>TGRPEWIWLALGTALMGLGTLYFLVKGMGVSDPDAKKFYAISTLVPAIAFTMYLSMLLGYGLTMVPFGGEQNPIYWARYADWLFTTPLLLLDLALLVDADQGTILALVGADGIMIGTGLVGALTKVYSYRFVWWAISTAAMLYILYVLFFGFTSKAESMRPEVASTFKVLRNVTVVLWSAYPVVW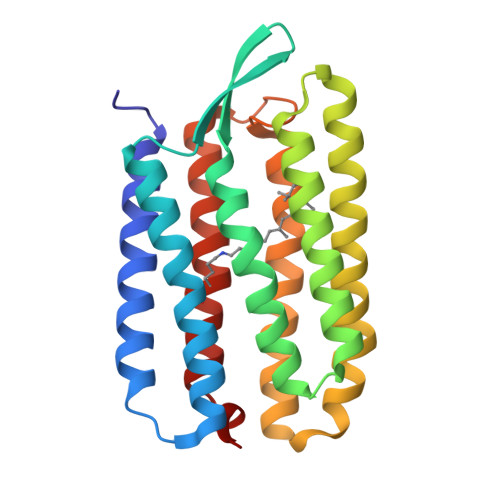LIGSEGAGIVPLNIETLLFMVLDVSAKVGFGLILLRSRAIFG[2x]> GPGSEFSDDSLVDYGEGGEGQFNEDGSFIGQYTVGSLVPRGSNDITPLHVASKRGNANMVKLLLDRGAKIDAKTRDGLTPLHCGARSGHEQVVEMLLDRAAPILSKTKNGLSPLHMATQGDHLNCVQLLLQHNVPVDDVTNDYLTALHVAAHCGHYKVAKVLLDKKANPNAKALNGFTPLHIACKKNRIRVMELLLKHGASIQAVTESGLTPIHVAAFMGHVNIVSQLMHHGASPNTTNVRGETALHMAARSGQAEVVRYLVQDG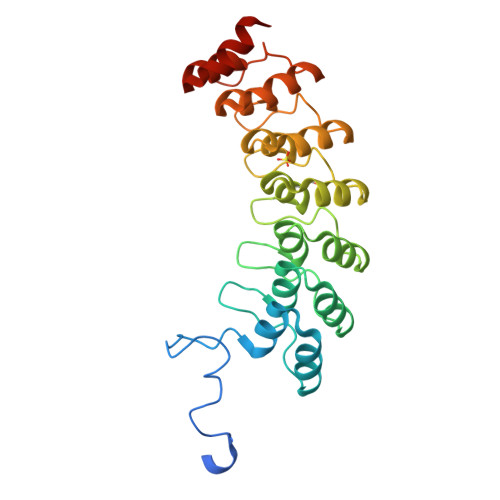AQV> MLPQPNSQVEQILAEFQLQEEDLKKVMRRMQKEMDRGLRLETHEEASVKMLPTYVRSTPEGSEVGDFLSLDLGGTNFRVMLVKVGEGEEGQWSVKTKHQMYSIPEDAMTGTAEMLFDYISECISDFLDKHQMKHKKLPLGFTFSFPVRHEDIDKGILLNWTKGFKASGAEGNNVVGLLRDAIKRRGDFEMDVVAMVNDTVATMISCYYEDHQCEVGMIVGTGCNACY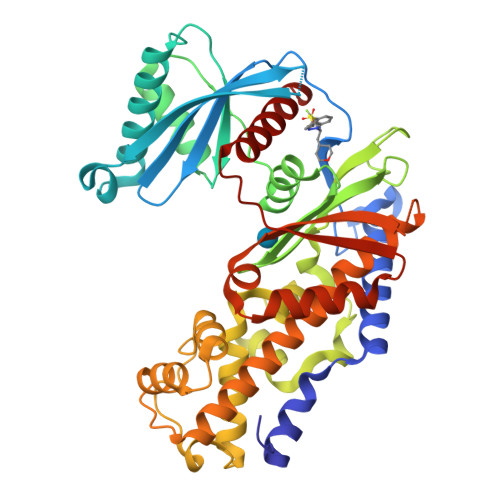MEEMQNVELVEGDEGRMCVNTEWGAFGDSGELDEFLLEYDRLVDESSANPGQQLYEKLIGGKYMGELVRLVLLRLVDENLLFHGEASEQLRTRGAFETRFVSQVESDTGDRKQIYNILSTLGLRPSTTDCDIVRRACESVSTRAAHMCSAGLAGVINRMRESRSEDVMRITVGVDGSVYKLHPSFKERFHASVRRLTPSCEITFIESEEGSGRGAALVSAVACKKACMLGQ The manganese transport regulator (MntR) functions as a homodimer and is activated by Mn2+ to repress the expression of two manganese uptake systems, MntABCD and MntH, in response to elevated concentrations of Mn2+. The MntR homologue (BH2807, BhMntR) in Bacillus halodurans is a protein consisting of 139 amino acids, and has 78% sequence identity with MntR from B.subtilis (BsMntR). Each BhMntR subunit was composed of seven α-helices and two β-strands, which could be divided into an N-terminal Helix-Turn-Helix (HTH) DNA binding domain (domain1, residues 1–71) and a C-terminal dimerization domain (domain2, residues 72–139). To further understand the metal binding site of the MntR protein, we determined crystal structures of the apo and manganese-bound forms of MntR from B. halodurans.

Mn2+-bound BhMntR crystals were obtained by soaking with 50 mM MnCl2 for one hour in apo crystals. The crystal structure of the Mn2+-bound form was determined at 2.5 Å resolution, and the binuclear manganese ions were clearly evident in the 2Fo-Fc map and omit maps, whereas a magnesium ion was observed in the other subunit. The two manganese ions were found at the interface between the HTH domain and the dimerization domain and formed a binuclear complex separated by 4.5 Å, labeled as the A and C sites (AC conformer). The binuclear manganese ions were liganded by six amino acid residues: Asp8 and Glu11 contributed by domain 1, and His 77, Glu99, Glu102, and His103 contributed by domain 2. The MnA ion was coordinated by seven atoms: Glu11 Oε1/Oε2, His77 Nδ1, Glu99 Oε2, Glu102 Oε1/Oε2, and Wat95 O. In addition, the His77 Nε2 made a hydrogen bond with Glu81 Oε1, while the His77 Nδ1 in the other subunit made a hydrogen bond with Glu81 Oε1 via a water molecule. The Mnc ion was coordinated by five atoms: Asp8 Oδ1, Glu99 Oε1, Glu102 Oε2, His103 Nε2, and Wat37 O, while the C site of BsMntR has octahedral coordination geometry. However, the other subunit contained a magnesium ion which was coordinated by the side chains of Glu99, Glu102, and two water molecules. The side chain of His77, which is strictly conserved in the MntR/IdeR family, had a different rotamer with a hydrogen bond via a water molecule to Glu81 and was also stabilized by π-π interaction with symmetry-related Tyr57. These interactions could block the proper rotamer of His77 to coordinate with MnA ion in this subunit. There were few structural differences between apo and Mn2+-bound dimeric forms, with a r.m.s.d. value of 0.49 Å for 276 Cα atoms.

>MPTPSMEDYLERIYLLIEEKGYARVSDIAEALEVHPSSVTKMVQKLDKSDYLVYERYRGLILTAKGKKIGKRLVYRHDLLEDFLKMIGVDSDHIYEDVEGIEHHLSWDAIDRIGDLVQYFQEDPSRLNDLREVQKKNEE[2x]>[2x]MAPITAYSQQTRGLL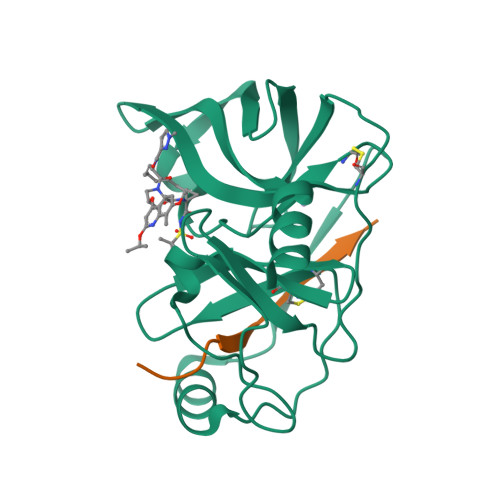GCIITSLTGRDKNQVDGEVQVLSTATQSFLATCVNGVCWTVYHGAGSKTLAGPKGPITQMYTNVDQDLVGWPAPPGARSMTPCTCGSSDLYLVTRHADVIPVRRRGDSRGSLLSPRPVSYLKGSSGGPLLCPSGHVVGIFRAAVCTRGVAKAVVFIPVESMETTMRASKKKK;>[2x]KKGSVVIVGRIILSGRK> MDGMKRTELDMYDDIFAVLERFPNVHNPHRVRIRRVGTKYFIEMDIEVDGKMSVKDAHELTVKIRKEMLKRRDDIEDVTIHVEPLGNVEE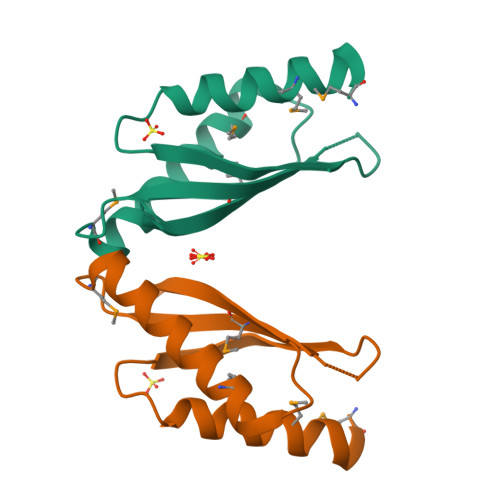EGFGLKKGEKKHHHHHH>[2x]MCKNEARLANELIEFVAATVTGIKNSPKENEQAFIDYLHCQYLERFQFFLGLLDGREFDTLFVFLFEELDRTIVTIDIGEEAIYDANLANKKYSTLLIIKSRSVIVDAEPIATQISAIYLPGPVNAGNLASIITHGVSSVFGQLIKS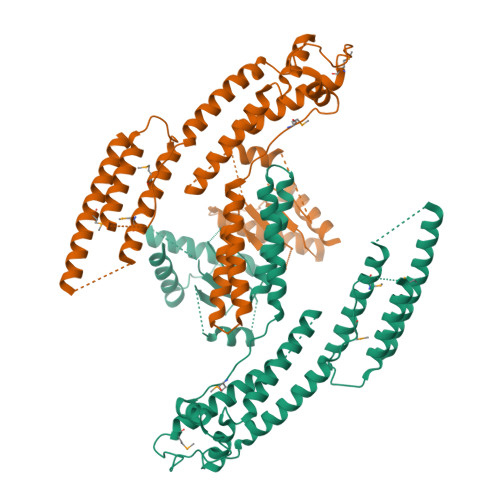DTKTYSVETIDKTRRKLDDISKQFQQLHTSIETPDLLAMVPSIIKLAVSKGATSHDYANYLPSNDLESMRFLNILQSIANKWFLVLKQTLAIDRDIKNGSFLDEVEFWSNFYEVLKSLIEQTQSQEFQVCLSVLTNAKRFHNLTNLLNEGSLSDKFKLADKYNQFLSSIPIDEVRQASNLEDLQELFPVLASSLKKFRYSGYPVQRFVVLMDKISQEVMDAILSNLSDLFQLEYGSFLGLYEKSAGMIEEWDDIVQDVNLLIREDLRKRAPQELLIQKLTFTSASVKATLDEILSTRKRFFSLAETIKSISPSTYHEEIQRLYHPFEQIHDISVNFRLKLEQAESEFSKNMLDLEKKLQNTLASFMDSDHCPTEKLSYLVKFKPLMELCPRIKVKVLENQQILLLEIKKD> MAHHHHHHMVHITLDPDTANPWLILSE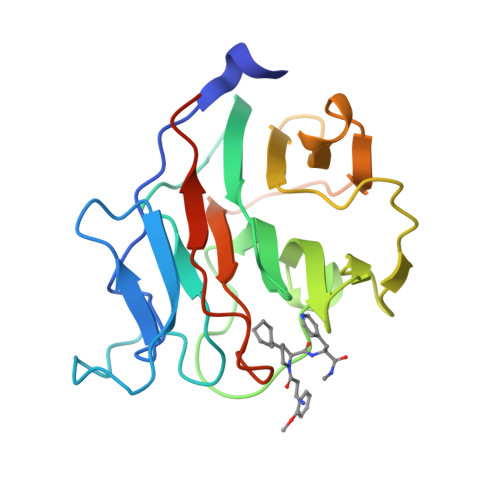DRRQVRLGDTQQSIPGNEERFDSYPMVLGAQHFHSGKHYWEVDVTGKEAWDLGVCRDSVRRKGHFLLSSKSGFWTIWLWNKQKYEAGTYPQTPLHLQVPPCQVGIFLDYEAGMVSFYNITDHGSLIYSFSECAFTGPLRPFFSPGFNDGGKNTAPLTLCPLNIGSQGSTDY In the early stage of eukaryotic DNA replication, the template DNA is unwound by the MCM helicase, which is activated by forming a complex with the Cdc45 and GINS proteins. On the other hand, the archaeal GINS appears to be either a tetramer formed by two types of subunits in a 2:2 ratio (α2β2) or a homotetramer of a single subunit (α4). The GINS complex from Pyrococcus furiosus increases the cognate MCM helicase activity, in a similar manner to eukaryotic GINS, in spite of the lack of a eukaryotic Cdc45 homolog. In this paper, we report the crystal structure of the α2β2 GINS tetramer from Thermococcus kodakaraensis (TkoGINS), which consists of the Gins51 and Gins23 subunits.

The crystal structure of TkoGINS was determined by the multiple isomorphous replacement method with anomalous dispersion (MIRAS), and the atomic model was refined at 2.65 Å. The crystal contains one pair of the Gins51 and Gins23 subunits in the asymmetric unit, and the protein forms the α2β2 tetramer generated by the crystallographic two-fold symmetry operation. Gins51 is composed of the larger α-helical domain at the N-terminus, and the smaller β-stranded domain at the C-terminus. In the Gins51 subunit, the long linker region between the two domains is disordered in the crystal, and 16 residues could not be assigned in the electron density map. Gins23 also possesses similar structural domains as in Gins51, but the order of the two domains in the sequence is permutated. The crystal structures of the TkoGINS tetramers revealed a stack of a two-fold symmetric dimer of the AB-type subunits (TkoGins51) onto another two-fold symmetric dimer of BA-type subunits (TkoGins23). The overall fold of each subunit and the tetrameric assembly of TkoGINS are essentially similar to those of human GINS. However, the locations of the C-terminal small domains are strikingly different between the two GINS, thus resulting in the formation of different subunit contacts in the complexes. Thus, to determine whether the Gins51 B domain is required for the stable tetramer formation, we examined the oligomeric state of a TkoGINS truncation mutant, lacking the B domain of Gins51, by gel filtration. This truncation mutant forms a stable tetramer, establishing that the C-terminal B domain of Gins51 is not essential for stable tetramer formation. However, a tryptophan residue is notably conserved among TkoGins23 (Trp30) and human Psf2 (Trp47) and Psf3 (Trp71) in this area.

> MDIVKLRELLEAELSSTDLNELDEDFYVEFDSLIKALKLSAESSRERGEDVEERLYLAQLKIAESLMKEIIKLRLHKIVDLAVEGKIAEMTAEEKRLFNVIRAFIEREELPEISEEVQPQEESEAEAEYRSKEVPKEAYIIQIDLPAVLGPDMKEYGPFMAGDMAIIPTVIGRALVEREAARRVRIFL;> NYFQGSHMFTGKALIAVKVMKPFGDWKSGDIVLVEDWKARELWEAGVVEIVDETDKIIGEIDKVIAEERESEPLTLLPEGLYERAEFYAYYLENYVRLNPRESVDTINVKLTKLANLRKKLRDLKLIRFNKILKAVMLRPNSLELLSRLAPEERRIYLQMSKIRNEWLGDA>MGSDKIHHHHHHMNESERKIV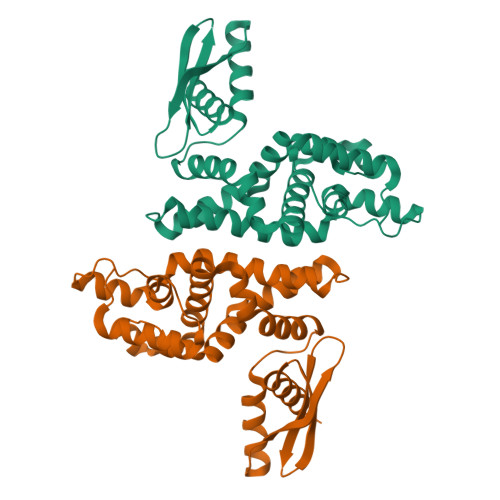EEFQKETGINFKNEELLFRALCHSSYANEQNQAGRKDVESNEKLEFLGDAVLELFVCEILYKKYPEAEVGDLARVKSAAASEEVLAMVSRKMNLGKFLFLGKGEEKTGGRDRDSILADAFEALLAAIYLDQGYEKIKELFEQEFEFYIEKIMKGEMLFDYKTALQEIVQSEHKVPPEYILVRTEKNDGDRIFVVEVRVNGKTIATGKGRTKKEAEKEAARIAYEKLLKERS[2x]> MTGSNSHITILTLNINGLNSAIKRHRLASWIKSQDPSVCCIQETHLTCRDTHRLKIKGWRKIYQANGKQKKAGVAILVSDKTDFKPTKIKRDKEGHYIMVKGSIQQEELTILNIYAPNTGAPRFIKQVLSDLQRDLDSHTLIMGDFNTPLSTLDRSTRQKVNKDTQELNSALHQADLIDIY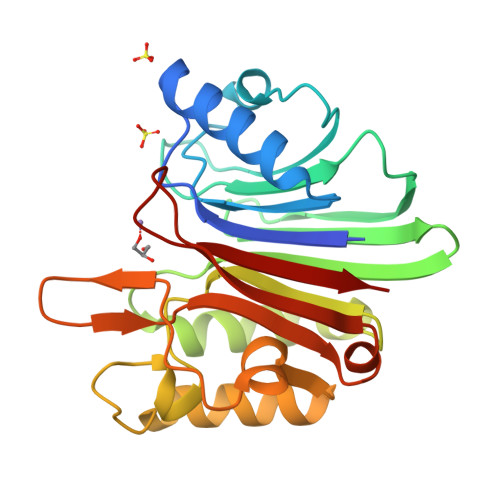RTLHPKSTEYTFSTANGESKIDHIVGSKALLSKCKRTEIITNYLSDHSAIKLELR> MEPKTKKQRSLYIPYAGPVLLEFPLLNKGSAFSMEERRNFNLLGLLPEVVETIEEQAERAWIQYQGFKTEIDKHIYLRNIQDTNETLFYRLVNNHLDEMMPVIYTPTVGAACERFSEIYRRSRGVFISYQNRHNMDDILQNVPNHNIKVIVVTDGERILGLGDQGIGGMGIPIGKLSLYTACGGISPAYTLPVVLDVGTNNQQLLNDPLYMGWRNPRITDDEYYEFVDEFIQAVKQRWPDVLLQFEDFAQKNAMPLLNRYRNEICSFNDDIQGTAAVTVGTLIAASRAAGGQLSEKKIVFRGAGSAGCGIAEMIISQTQREGLSEEAARQKVFMVDRFGLLTDKMPNLLPFQTKLVQKRENLSDWDTDSDVLSLLDVVRNVKPDILIGVSGCTGLFTEEIIREMHKHCPRPI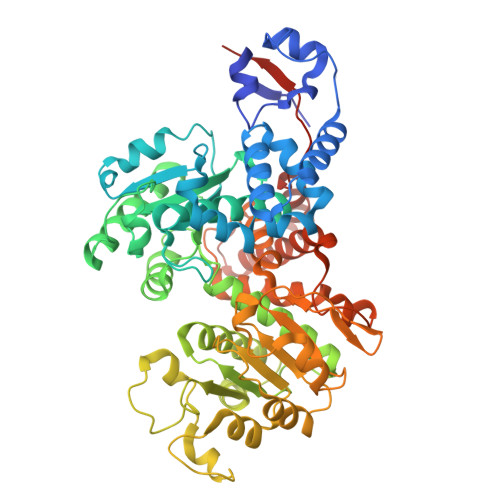VMPLSNPTSRVEATPQDIIAWTEGNALVATGSPFNPVVWKDKIYPIAQCNNAFIFPGIGLGVIASGASRITDEMLMSASETLAQYSPLVLNGEGMVLPELKDIQKVSRAIAFAVGKMAQQQGVAVKTSAEALQQAIDDNFWQAEYRDYRRTSILEHHHHHH>[2x]SSKVSEQLKCCSGILKEMFAKKHAAYAWPFYKPVDVE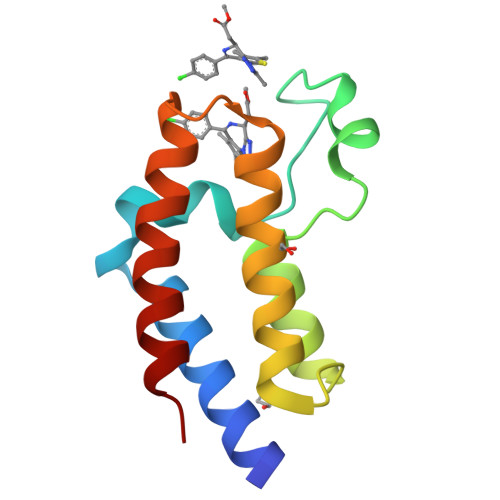ALGLHDYCDIIKHPMDMSTIKSKLEAREYRDAQEFGADVRLMFSNCYKYNPPDHEVVAMARKLQDVFEMRFAKMP1-ethanoylpiperidine-4-carbonitrile | C8 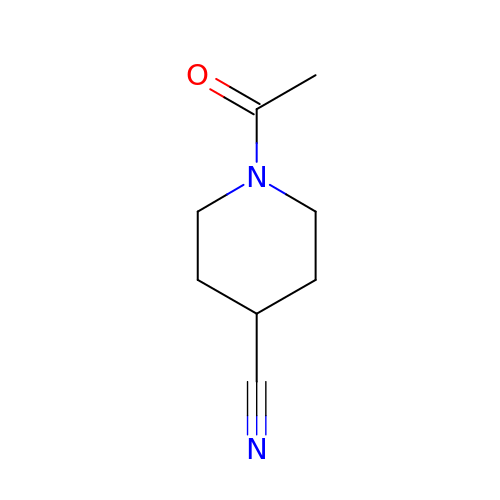H12 N2 O | NFDGRMQIOHRQHF-UHFFFAOYSA-N>MGHHHHHHMGTGLQEQQMSRGDIPIIVDACISFVTQHGLRLEGVYRKGGARARSLRLLAEFRRDARSVKLRPGEHFVEDVTDTLKRFFRELDDPVTSARLLPRWREAAELPQKNQRLEKYKDVIGCLPRVNRR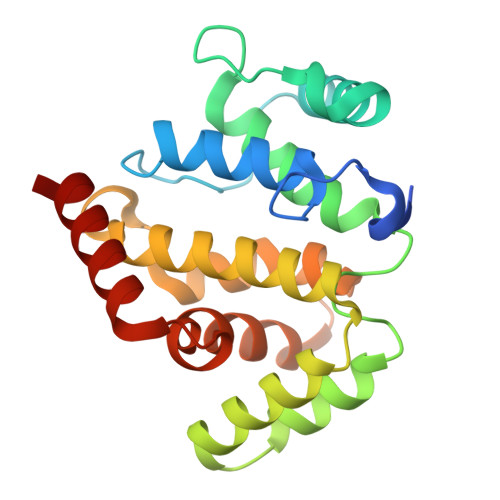TLATLIGHLYRVQKCAALNQMCTRNLALLFAPSVFQTDGRGEHEVRVLQELIDGYISVFDIDSDQVAQIDLEVSLITT[2x]6-CHLORO-N-((3S)-2-OXO-1-{4-[(2R)-2--PYRROLIDINYL] 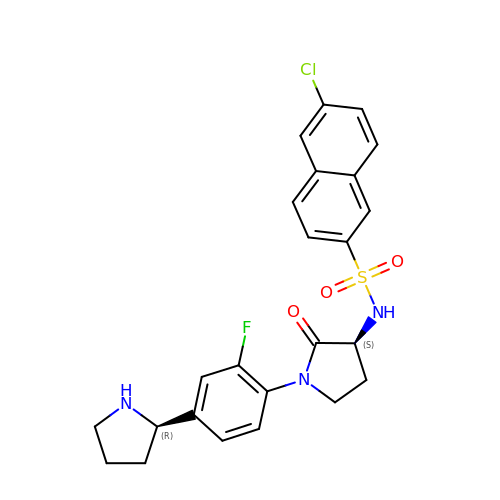PHENYL}-3-PYRROLIDINYL)-2-NAPHTHALENESULFONAMIDE | C24 H23 Cl F N3 O3 S | OKMBULRSJZKGQF-YADHBBJMSA-N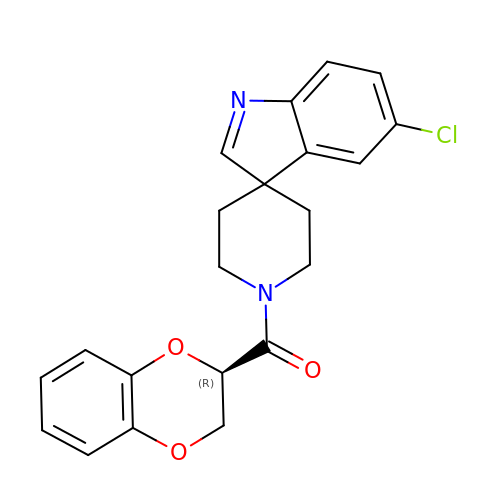(5-chloro-1'H-spiro[indole-3,4'-piperidin]-1'-yl)[(2R)-2,3-dihydro-1,4-benzodioxin-2-yl]methanone | C21 H19 Cl N2 O3 | FORRKPPZDDUANL-LJQANCHMSA-N> PFIECHIATGLSVARKQQLIRDVIDVTNKSIGSDPKIINVLLVEHAEANMSISGRIHG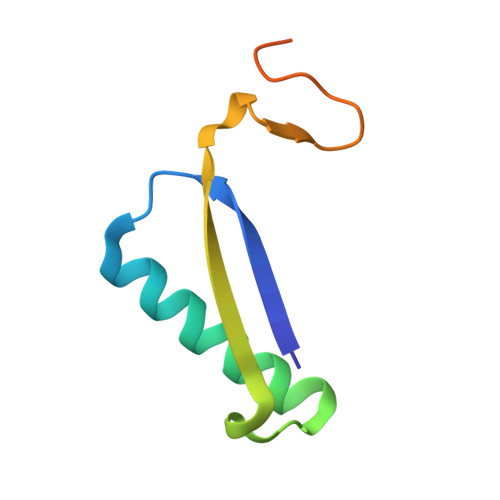EAASTERTPAVS>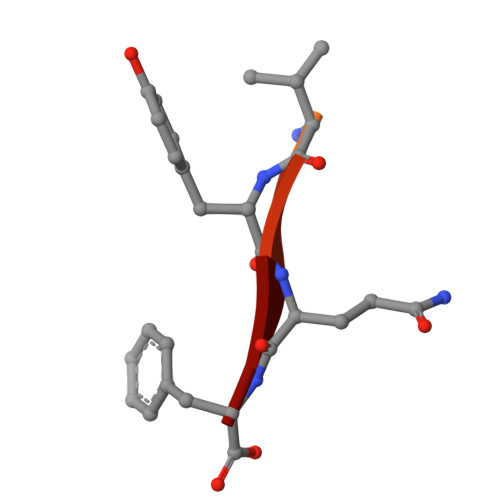 DNRDGNVYQF>[8x]GMEPFKQQKVEDFYDIGEELGSGQFAIVKKCREKSTGLEYAAKFIKKRQSRASRRGVSREEIEREVSILRQVLHHNVITLHDVYENRTDVVLILELVSGGELFDFLAQKESLSEEEATSFIKQILDGVNYLHTKKIAHFDLKPENIMLLDKNIPIPHIKLIDFGLAHEIEDGVEFKNIFGTPEFVAPEIVNYEPLGLEADMW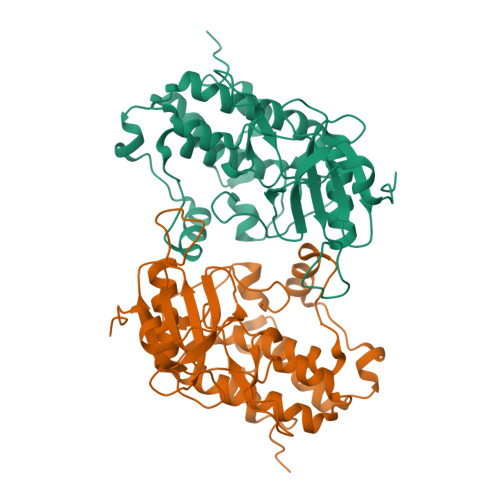SIGVITYILLSGASPFLGDTKQETLANITSVSYDFDEEFFSHTSELAKDFIRKLLVKETRKRLTIQEALRHPWITPVDNQQAMVRR> HHAADYVLYKDATKPVEDRVADLLGRMTLAEKIGQMTQIERLVATPDVLRDNFIGSLLSGGGSVPRKGATAKEWQDMVDGFQKACMSTRLGIPMIYGIDAVHGQNNVYGATIFPHNVGLGATRDPYLVKRIGEATALEVRATGIQYAFAPCIAVCRDPRWGRCYESYSEDRRIVQSMTELIPGLQGDVPKDFTSGMPFVAGKNKVAACAKHFVGDGGTVDGINENNTIINREGLMNIHMPAYKNAMDKGVSTVMISYSSWNGVKMHANQDLVTGYLKDTLKFKGFVISDYEGIDRITTPAGSDYSYSVKASILAGLDMIMVPNKYQQFISILTGHVNGGVIPMSRIDDAVTRILRVKFTMGLFENPYADPAMAEQLGKQEHRDLAREAARKSLVLLKNGKTSTDAPLLPLPKKAPKILVAGSHADNLGYQCGGWTIEWQGDTGRTTVGTTILEAVKAAVDPSTVVVFAENPDAEFVKSGGFSYA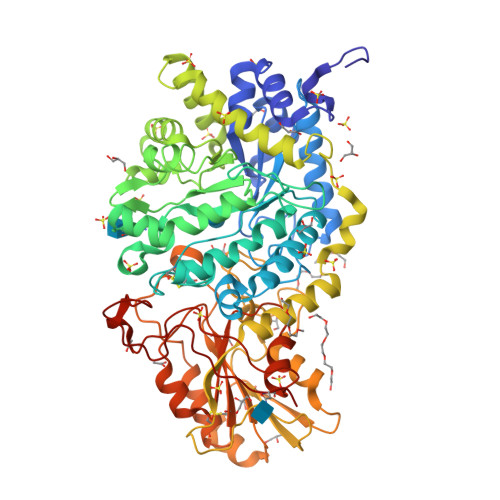IVAVGEHPYTETKGDNLNLTIPEPGLSTVQAVCGGVRCATVLISGRPVVVQPLLAASDALVAAWLPGSEGQGVTDALFGDFGFTGRLPRTWFKSVDQLPMNVGDAHYDPLFRLGYGLTTNATKKY> AMAEMKTDAATLAQEAGNFERISGDLKTQIDQVESTAGSLQGQWRGAAGTA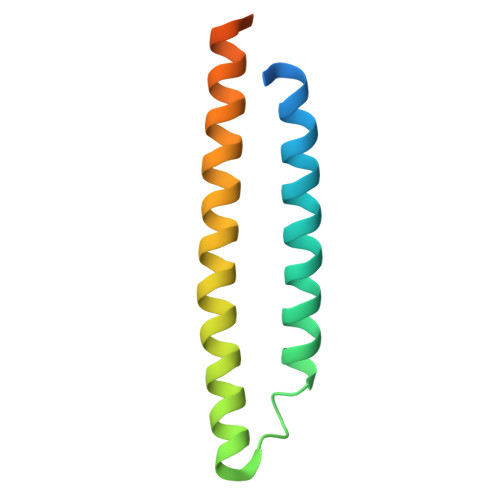AQAAVVRFQEAANKQKQELDEISTNIRQAGVQYSRADEEQQQALSSQMGF> AQRGAGAGAAEPGPPRTPRPGRREPVMPRPPVPANALGARGEAVRLQLQGEELRLQEESVRLHQINIYLSDRISLHRRLPERWNPLCKEKKYDYDNLPRTSVIIAFYNEAWSTLLRTVYSVLETSPDILLEEVILVDDYSDREHLKERLANELSGLPKVRLIRANKREGLVRARLLGASAARGDVLTFLDCHCECHEGWLEPLLQRIHEEESAVVCPVIDVIDWNTFEYLGNSGEPQIGGFDWRLVFTWHTVPERERIRMQSPVDVIRSPTMAGGLFAVSKKYFEYLGSYDTGMEVWGGENLEFSFRIWQCGGVLETHPCSHVGHVFPKQAPYSRNKALANSVRAAEVWMDEFKELYYHRNPRARLEPFGDVTERKQLRDKLQCKDFKWFLETVYPELHVPEDRPGFFGMLQNKGLTDYCFDYNPPDENQIVGHQVILYLCHGMGQNQFFEYTSQKEIRYNTHQPEGCIAVEAGMDTLIMHLCEETAPENQKFILQEDGSLFHEQSK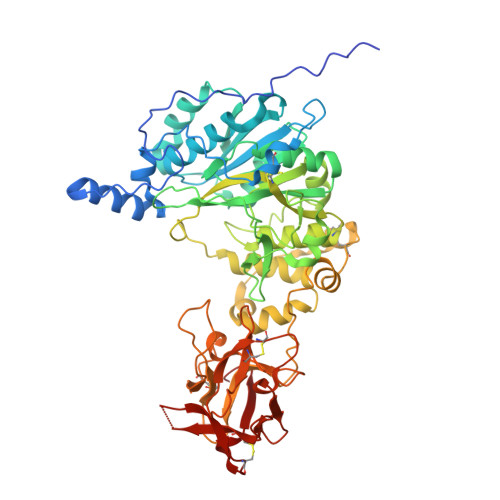KCVQAARKESSDSFVPLLRDCTNSDHQKWFFKERML>[2x]MLYIDEFKEAIDKGYILGD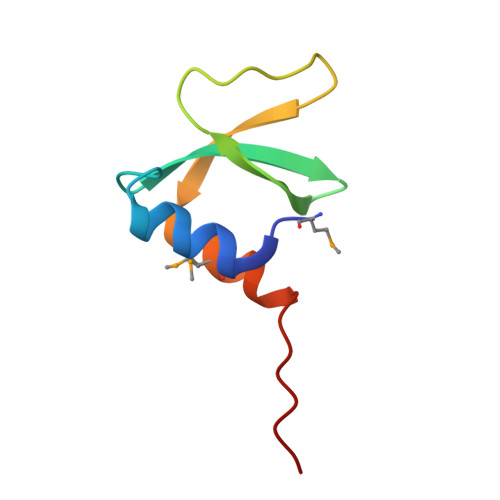TVAIVRKNGKIFDYVLPHEKVRDDEVVTVERVEEVMVELDKLEHHHHHH>[2x]MKQLSVSLAILCAVATSEAFAADELQQRAQGLFKPVPAKAPTLKGNPASPVKVELGKMLYFDPRLSASHLISCNTCHNVGLGGGDLQATSTGHGWQKGPRNAPTVLNSVFNTAQFWDGRAKDLAEQAKGPVQAPVEMNNTPDQVVKTLNSIPDYVALFKKAFPGEKDPVTFDNMAKAIEVFEATLITPDSPFDQYLKGKKKALDGKQTAGLKLFLDKGCVACHGGLNLGGTGYFPFGVVEKPAE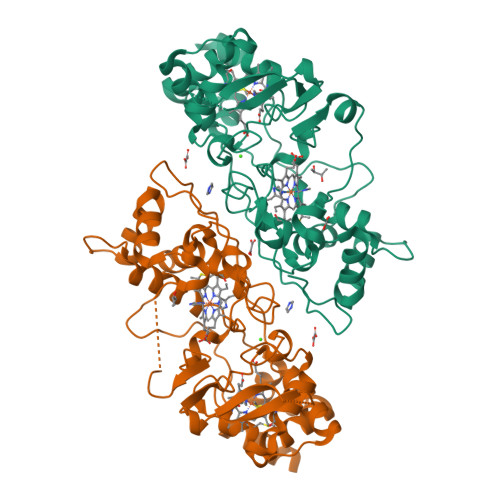NILPLGDKGRFAVTNTAKDEYVFRAPSLRNVAITYPYFHSGVVWSLKEAVAVMGSAQFGIKLSDDESEAIAAFLGSLTGKQPKVVYPIMPASTDATPRPRL>[4x]KE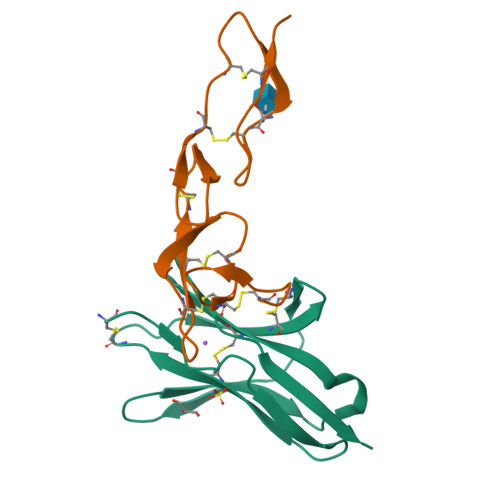SCDVQLYIKRQSEHSILAGDPFELECPVKYCANRPHVTWCKLNGTTCVKLEDRQTSWKEEKNISFFILHFEPVLPNDNGSYRCSANFQSNLIESHSTTLYVTDVK;>EICKPEEVQLGDQCCPPCKQGYRVTGQCTQYTSTTCTLCPSGTYVSGLYQCTQCTECQDTEVTIRNCTSTQNTVCASKQYTSFSVPGVQHHKQRQSHTAHVTVKQGKSGRHTHHHHHH[4x]>[2x]AEVTQLSNGIVVATEHNPSAHTASVGVVFGSGAANENPYNNGVSNLWKNIFLSKENSAVAAKEGLALSSNISRDFQSYIVSSLPGSTDKSLDFLNQSFIQQKANLLSSSNFEATKKSVLKQVQDFEENDHPNRVLEHLHSTAFQNTPLSLPTRGTLESLENLVVADLESFANNHFLNSNAVVVGTGNIKHEDLVNSIESKNLSLQTGTKPVLKKKAAFLGSEVRLRDDTLPKAWISLAVEGEPVNSPNYFVAKLAAQIFGSYNAFEPASRLQGIKLLDNIQEYQLCDNFNHFSLSYKDSGLWGFSTATRNVTMIDDLIHFTLKQWNRLTISVTDTEVERAKSLLKLQLGQLYESGNPVNDANLLGAEVLIKGSKLSLGEAFKKIDAITVKDVKAWAGKRLWDQDIAIAGTGQIEGLLDYMRIRSDMSMMRW;>LTVSARDAPTKISTLAVKVHGGSRYATKDGVAHLLNRFNFQNTNTRSALKLVRESELLGGTFKSTLDREYITLKATFLKDDLPYYVNALADVLYKTAFKPHELTESVLPAARYDYAVAEQCPVKSAEDQLYAITFRKGLGNPLLYDGVERVSLQDIKDFADKVYTKENLEVSGENVVEADLKRFVDESLLSTLPAGKSLVSKSEPKFFLGEENRVRFIGDSVAAIGIPVNKASLAQYEVLANYLTSALSELSGLISSAKLDKFTDGGLFTLFVRDQDSAVVSSNIKKIVADLKKGKDLSPAINYTKLKNAVQNESVSSPIELNFDAVKDFKLGKFNYVAVGDVSNLPYLDEL[2x];>MAFRKSNVYLSLVNSYIIDSPQPSSINYWWNMGSLLGLCLVIQIVTGIFMAMHYSSNIELAFSSVEHIMRDVHNGYILRYLHANGASFFFMVMFMHMAKGLYYGSYRSPRVTLWNVGVIIFILTIATAFLGYCCVYGQMSHWGATVITNLFSAIPFVGNDIVSWLWGGFSVSNPTIQRFFALHYLVPFIIAAMVIMHLMALHIHGSSNPLGITGNLDRIPMHSYFIFKDLVTVFLFMLILALFVFYSPNTLGHPDNYIPGNPLVTPASIVPEWYLLPFYAILRSIPDKLLGVITMFAAILVLLVLPFTDRSVVRGNTFKVLSKFFFFIFVFNFVLLGQIGACHVEVPYVLMGQIATFIYFAYFLIIVPVISTIENVLFYIGRVNK[2x];>MTAAEHGLHAPAYAWSHNGPFETFDHASIRRGYQVYREVCAACHSLDRVAWRTLVGVSHTNEEVRNMAEEFEYDDEPDEQGNPKKRPGKLSDYIPGPYPNEQAARAANQGALPPDLSLIVKARHGGCDYIFSLLTGYPDEPPAGVALPPGSNYNPYFPGGSIAMARVLFDDMVEYEDGTPATTSQMAKDVTTFLNWCAEPEHDERKRLGLKTVIILSSLYLLSIWVKKFKWAGIKTRKFVFNPPKPRK[2x];>[2x]KSTYRTPNFDDVLKENNDADKGRSYAYFMVGAMGLLSSAGAKSTVETFISSMTATADVLAMAKVEVNLAAIPLGKNVVVKWQGKPVFIRHRTPHEIQEANSVDMSALKDPQTDADRVKDPQWLIMLGICTHLGCVPIGEAGDFGGWFCPCHGSHYDISGRIRKGPAPLNLEIPAYEFDGDKVIVG;>MGMLELVGEYWEQLKITVVPVVAAAEDDDNEQHEEKAAEGEEKEEENGDEDEDEDEDEDDDDDDDEDEEEEEEVTDQLEDLREHFKNTEEGKALVHHYEECAERVKIQQQQPGYADLEHKEDCVEEFFHLQHYLDTATAPRLFDKLK[2x];>[2x]MPQSFTSIARIGDYILKSPVLSKLCVPVANQFINLAGYKKLGLKFDDLIAEENPIMQTALRRLPEDESYARAYRIIRAHQTELTHHLLPRNEWIKAQEDVPYLLPYILEAEAAAKEKDELDNIEVSK;>GPPSGKTYMGWWGHMGGPKQKGITSYAVSPYAQKPLQGIFHNAVFNSFRR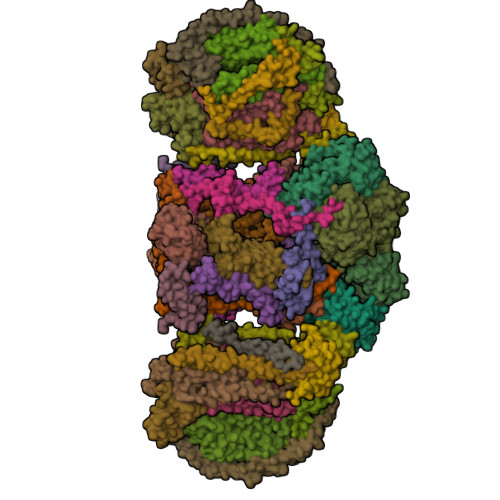FKSQFLYVLIPAGIYWYWWKNGNEYNEFLYSKAGREELERVNV[2x];>[2x]MSFSSLYKTFFKRNAVFVGTIFAGAFVFQTVFDTAITSWYENHNKGKLWKDVKARIAAGDGDDDDE;>MAYTSHLSSKTGLHFGRLSLRSLTAYAPNLMLWGGASMLGLFVFTEGWPKFQDTLYKKIPLLGPTLEDHTPPEDKPN[2x];>MVQRWLYSTNAKDIAVLYFMLAIFSGMAGTAMSLIIRLELAAPGSQYLHGNSQLFNVLVVGHAVLMIFFLVMPALIGGFGNYLLPLMIGATDTAFPRINNIAFWVLPMGLVCLVTSTLVESGAGTGWTVYPPLSSIQAHSGPSVDLAIFALHLTSISSLLGAINFIVTTLNMRTNGMTMHKLPLFVWSIFITAFLLLLSLPVLSAGITMLLLDRNFNTSFFEVSGGGDPILYEHLFWFFGHPEVYILIIPGFGIISHVVSTYSKKPVFGEISMVYAMASIGLLGFLVWSHHMYIVGLDADTRAYFTSATMIIAIPTGIKIFSWLATIHGGSIRLATPMLYAIAFLFLFTMGGLTGVALANASLDVAFHDTYYVVGHFHYVLSMGAIFSLFAGYYYWSPQILGLNYNEKLAQIQFWLIFIGANVIFFPMHFLGINGMPRRIPDYPDAFAGWNYVASIGSFIATLSLFLFIYILYDQLVNGLNNKVNNKSVIYNKAPDFVESNTIFNLNTVKSSSIEFLLTSPPAVHSFNTPAVQS[2x];>[2x]DVPTPYACYFQDSATPNQEGILELHDNIMFYLLVILGLVSWMLYTIVMTYSKNPIAYKYIKHGQTIEVIWTIFPAVILLIIAFPSFILLYLCDEVISPAMTIKAIGYQWYWKYEYSDFINDSGETVEFESYVIPDELLEEGQLRLLDTDTSMVVPVDTHIRFVVTAADVIHDFAIPSLGIKVDATPGRLNQVSALIQREGVFYGACSELCGTGHANMPIKIEAVSLPKFLEWLNEQ;>MTHLERSRHQQHPFHMVMPSPWPIVVSFALLSLALSTALTMHGYIGNMNMVYLALFVLLTSSILWFRDIVAEATYLGDHTMAVRKGINLGFLMFVLSEVLIFAGLFWAYFHSAMSPDVTLGACWPPVGIEAVQPTELPLLNTIILLSSGATVTYSHHALIAGNRNKALSGLLITFWLIVIFVTCQYIEYTNAAFTISDGVYGSVFYAGTGLHFLHMVMLAAMLGVNYWRMRNYHLTAGHHVGYETTIIYTHVLDVIWLFLYVVFYWWGV[2x];>QQKPVVKTAQNLAEVNGPETLIGPGAKEGTVPTDLDQETGLARLELLGKLEGIDVFDTKPLDSSRKGTMKDPIIIESYDDYRYVGCTGSPAGSHTIMWLKPTVNEVARCWECGSVYKLNPVGVPNDDHHH[2x];>[2x]AQTHALSNAAVMDLQSRWENMPSTEQQDIVSKLSERQKLPWAQLTEPEKQAVWYISYGEWGPRRPVLNKGDSSFIAKGVAAGLLFSVGLFAVVRMAGGQDAKTMNKEWQLKSDEYLKSKNANPWGGYSQVQSK;>[2x]SDAHDEETFEEFTARYEKEFDEAYDLFEVQRVLNNCFSYDLVPAPAVIEKALRAARRVNDLPTAIRVFEALKYKVENEDQYKAYLDELKDVRQELGVPLKEELFPSSS;>ANKVIQLQKIFQSSTKPLWWRHPRSALYLYPFYAIFAVAVVTPLLYIPNAIRGIKAKKA[2x];>VHFKDGVYENIPFKVKGRKTPYALSHFGFFAIGFAVPFVACYVQLKK[2x];>[2x]TIAPITGTIKRRVIMDIVLGFSLGGVMASYWWWGFHMDKINKREKFYAELAERKK;>ADQENSPLHTVGFDARFPQQNQTKHCWQSYVDYHKCVNMKGEDFAPCKVFWKTYNALCPLDWIEKWDDQREKGIFAGDINSD[2x];>ASSLPPNALKPAFGPPDKVAAQKFKESLMATEKHAKDTSNMWVKISVWVALPAIALTAVNTYFVEKEHAEHREHLKHVPDSEWPRDYEFMNIRSKPFFWGDGDKTLFWNPVVNRHIEHDDGARGSHHHHHH[2x];>MFFSQVLRSSARAAPIKRYTGGRIGESWVITEGRRLIPEIFQWSAVLSVCLGWPGAVYFFSKARKA[2x]> MRRHY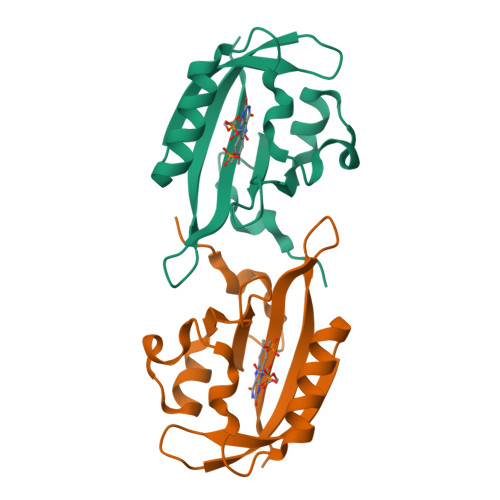RDLIRNTPMPDTPQDIADLRALLDEDEAEMSVVFSDPSQPDNPTIYVSDAFLVQTGYTLEEVLGRNCRFLQGPDTNPHAVEAIRQGLKAETRFTIDILNYRKDGSAFVNRLRIRPIYDPEGNLMFFAGAQNPVLEHHHHHH>[2x]MKKIKPHGPLPSQTQLAYLGDELAAFIHFGPNTFYDQEWGTGQEDPERFNPSQLDAREWVRVLKETGFKKLILVVKHHDGFVLYPTAHTDYSVKVSPWRRGKGDLLLEVSQAATEFDMDMGVYLSPWDAHSPLYHVDREADYNAYYLAQLKEILSNPNYGNAGKFAEVWMNGARGEGAQKVNYEFEKWFETIRDLQGDCLIFSTEGTSIRWIGNQRGYAGDPLWQKVNPDKLGTEAELNYL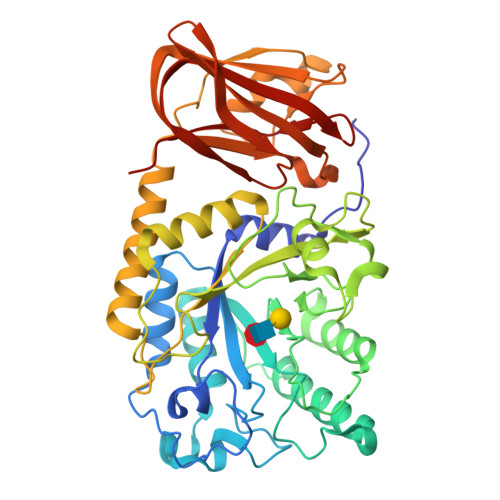QHGDPSGTIFSIGEADVSIRPGWFYHEDQDPKSLEELVEIYFHSVGRGTPLLLNIPPNQAGLFDAKDIERLYEFATYRNELYKEDLALGAEVSGPALSADFACRHLTDGLETSSWASDADLPIQLELDLGSPKTFDVIELREDLKLGQRIAAFHVQVEVDGVWQEFGSGHTVGYKRLLRGAVVEAQKIRVVITESQALPLLTKISLYKTP>MTPVAEGGLPHGSVPSLSHTRQWRPGVVQEVAPAGVLDLGPGYIEPALLPVRLLRGAYEQALAEYGAAALGYGHDPGAQPLRDRLAARAAAADGLPCDPDQVLLTSGTSQALYLLATSLAAPGDTVLTEELCYDLGQRIFRDCSLRLRQVAMDGSGMLPDALDRALTEGARAGAKTAFVYLTPTHHNPTGHTMPLARRRLLLEVAARHDVLIVEDDAYTELSLIPDRTPPPSLAALAGYRRVVRLCSFSKTLGPGLRLGWLLADRELAGRLATHGLFVSGGSLNHTTSLAVSTLLASGAYDRHLDAFRAQLRARRDALVGALRAMLDDGVELRTPEGGFFLWLRAGDGADERELLDGAARAGVRIAAGSRFGTTQGAGLRLAFSFNPPALLEQAAKRLTTAWSGSTPDLEIGVRS[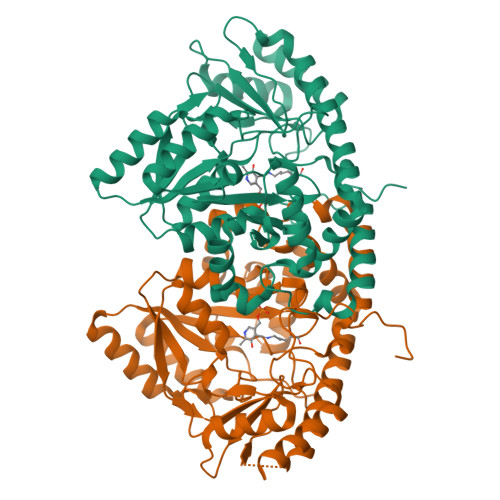2x]>MDSRPEFLNPIQTVSVLESAEPGTVIANITAIDHDLNPKLEYHIVGIVAKDDTDRLVPNQEDAFAVNINTGSVMVKSPMNRELVATYEVTLSVIDNASDLPERSVSVPNAKLTVNVLDVNDNTPQFKPFGITYYMERILEGATPGTTLIAVAAVDPDKGLNGLVTYTLLDLVPPGYVQLEDSSAGKVIANRTVDYEEVHWLNFTVRASDNGSPPRAAEIPVYLEIVDINDNNPIFDQPSYQEAVFEDVPVGTIILTVTATDADSGNFA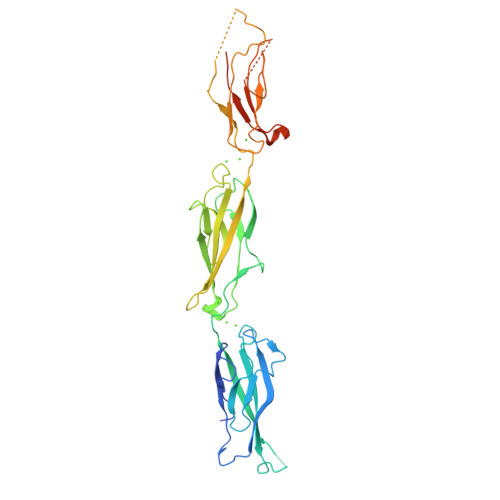LIEYSLGDGESKFAINPTTGDIYVLSSLDREKKDHYILTALAKDNPGDVASNRRENSVQVVIQVLDVNDCLEHHHHHH[2x]> MRAFSTLDRENETFVPSVRVYADGETEDNSFSLKYRSNWTPGRFNSTGAKTKQWHYPSPYSRGALSVTSIDQGAYKRSGSSWGRPYEEKAGFGFSLDARSCYSLFPVSQNLTYIEVPQNVANRASTEVLQKVTQGNFNLGVALAEARSTASQLATQTIALVKAYTAARRGNWRQALRYLALNEDRKFRSKHVAGRWLELQFGWLPLMSDIQGAYEMLTKVHLQEFLPMRAVRQVGTNIKLDGRLSYPAANFQTTCNISRRIVIWFYINDARLAWLSSLGILNPLGIVWEKVPFSFVVDWLLPVGNMLEGLTAPVGCSYMSGTVTDVIT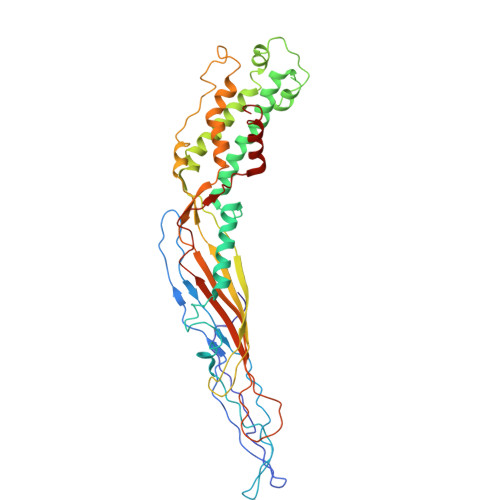GESIISVDAPYGWTVERQGTAKAQISAMHRGVQSVWPTTGAYVKSPFSMVHTLDALALIRQRLSR> GSHMLKGQEFAPSHQQVYAPLRADGDKPRAHLTVVRQTPTQHFKNQFPALHWEHELGLAFTKNRMNYTNKFLLIPESG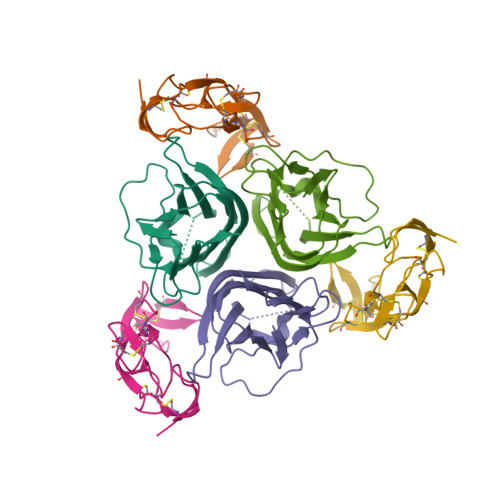DYFIYSQVTFRGMTSECSEIRQAGRPNKPDSITVVITKVTDSYPEPTQLLMGTKSVSEVGSNWFQPIYLGAMFSLQEGDKLMVNVSDISLVDYTKEDKTFFGAFLL;> RSVAETPTYPWRDAETGERLVCAQCPPGTFVQRPCRRDSPTTCGPCPPRHYTQFWNYLERCRYCNVLCGEREEEARACHATHNRACRCRTGFFAHAGFCLEHASCPPGAGVIAPGTPSQNTQCQPCPPGTFSASSSSSEQCQPHRNCTALGLALNVPGSSSHDTLCTSTGHHHHHH> XQLV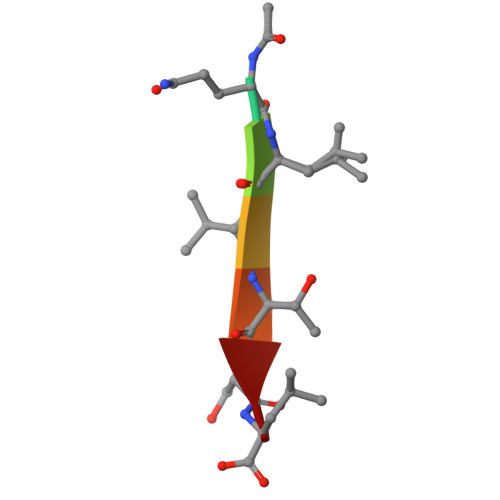TSL> QVYDKVVLRGESPLRWDGENHPLTFDESEGLWKSEPVTLSGGIQFEYKFVMDNEWLAGDNLRFQVPQTGDYVFYFD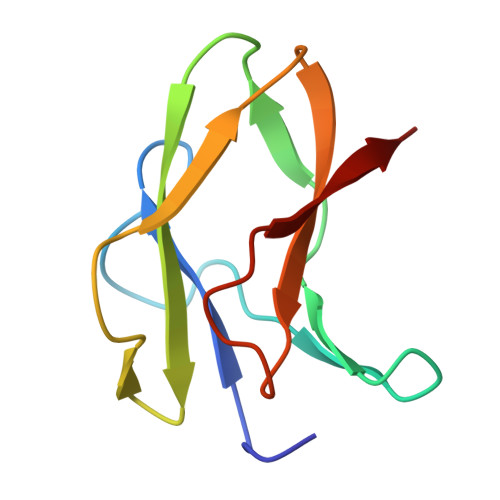PSDQRKVDVRPVT> MRARLFQSLAIQVAEEGLLTTALSGYACRAFSANGVTKFGFQCSSVSTSAASHEASSSRGSGDQGRVTGGRQERAGRQAPTGSDGPQRADRAKQGYADGGKSRSLFRRDNNPDSGSRGGDGQRGGGKGAGTGSGYSGGSSGQRGGPWQQQQGGRQHDRRGDDRRGGGGGGGPPPMLRDGRDGRDGRGGGGRPPFAPSGPGSGSRAPRAARWDALDVAASNAPQRLLQLVGDPRSGVADDTSSPAFGEVTVELLHHQPSNEVYWYKYAFAGGQPGGRGGHRDGRLSDYSRNLAYVLRAKDPARWSVEALADKFRVRPQRMLAALALKELEAQRLESGALLRGPLSAYSLRVSLADVHLDKASGAPRLRPASAPPAASRELLLGRMLPRVVSA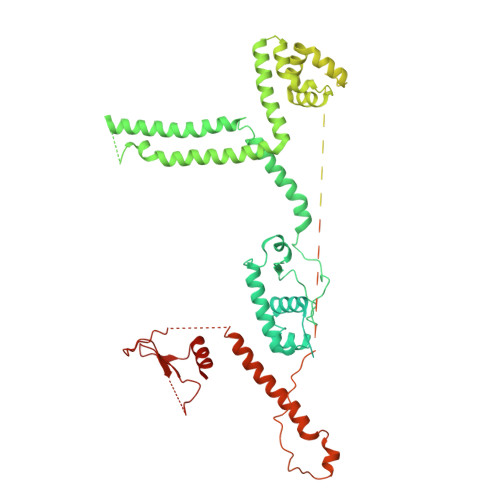TQRTQAALLSALRPHGFDAAALRAALQADVAAVEAAAGELDAAAAAAGGEGAEGGTAAGGVSAYLAPELAACRAAVEAVAAAVEVVVNASPLLQEERQAAALRARVEAALQAGAGQAPAAAAAVAGTGAGAGGGADGNSKDAVPAAAAAAATSPGGGEALEVLLQPLTQDGSGAPLQRFLFSLPPPIRVALLRQLPRLAAQLAAAGVDLQRAGRDAAYRGPLAPAAPAATPAGSKQQQQQRQKQGGAAASTRSGKLPRLTVDVLGFVPVSEAQAEALAAAVESAAAAEAALVAKLEALQVAAGAAPAPAAGAAAAAAAAAATAPSAAELRDARSLLRQYLSTHSMWGELRLAARKAAGHSPDTRGKRRKLEVMAEADPAALTRALQVEAHTQLRRSHDRAAAESLKAGVAAAAATEAAAAAAASGSEAAAKPPTPLSDPAGWDALAAWLDAEVAGRVYARGSGERLVVRLPTYPAFEGYPLSELDKAREGELGALNRLVAARTAAAQWAAFRRDLLFNLGVRGEKLRDNDLPGAPAWPANLRTELTRPVVVYGIGPDGATQYPPVYVAAGDGAKRPLNEQEKVYQERRLPGPRLPYHMGRIRTLPELN>MGSSHHHHHHHSSGLVPRGSHHMLEMQINLPEVHAEVTAQFVRYEKALTSNDTAVLNELFWNSPQTLRYGATENLYGYEAIAGFRATRSPNNLEREIVRTVITTYGHDFATANIEFRRLSHSQLTGRQSQTW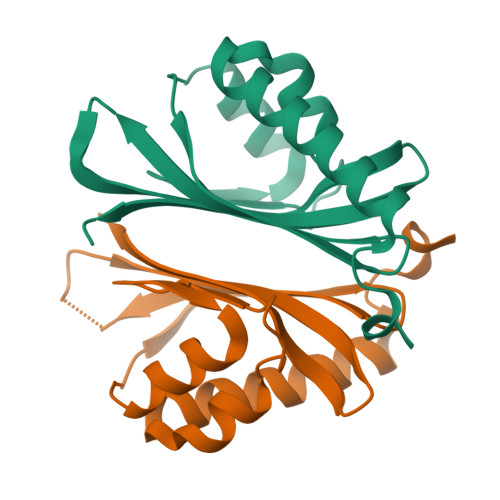MRTSQGWRVVAAHVSLIALPVS[4x]> MSLPIRNSIKRYKEQLKKPLFKNEALYQLTKLYLSLENEINENELDECKDYFNQLKQSGVLKESQKELKEITIDFQTITKQYDLAEQSLQSAIKSYPDNLNFLLKNINLLSINKKYYEFFKSIKDSKIKYQRDLKYLNFIIKQIDNVAIKAIKESVEEIQANTMLLNDSMSYLNLITLKTEILDYIIRATIHNNLVSSNSSGSIDDIDDIGDYYGNNNFNQKLTRQLKEFKKQVKKIRELVSLYKEPITLSPSLEEFNERYFFYKGILIDYEYSNISNITTSISNIKNRQNPPFKSYLKSLQKDITKSSSSNMLEPIVKLSSEVSRQLFYSINRIIGDGNEIDLKLNFYASLNNNINMNLNIGDSGMYKYLDYLVSKFNSVSSPNDTDQLDTLFIESIEKNDFQYLLNNPLEFQRFISFSLWHINKTSSYTTLICWLDKIFNKFINRINFELQQLSSKSSSSTTTTTTSSSSHITLLHIIVYCINLIFETDYQQDYQQQQKQQQQQQQQQSYQLSSLEVYLDSTLNVPFLRNSLPWKIWNSMIYYSNLKPSSKINSTEIFSITTLSELLNGILKNGDHLHPLTCYKIAKDLPMITQHYQNEVDLSQTDIDISKIQATYYLITLRHITYLNQQRQQQQQDNNNNNDINNNNNNNNQIIQDKNFLKNIENTCNHCLSDLYKDKQNLKGALQYLLKVDTPIAYVETIYLCRDIIYNNKSNPAYTRPVIQSLITLMNQVWNKCQDFNANDLDYYQVDHDEYLNDIDASLEIITKLKDQYNFYDVPSTPSSSSLYTTPTKPTTVVPFSSIYGNNYNNNNNNNNNSLISSTPQRGRLSLPSTSTPLKVSMLSNSPNKSNNNNNNNNKQIQQSQQNKSDLPKFNVVEEEEEEEEVDINSFKDVFLQRRKERAELLKTLSNKRKALVCPQEFNKPLRSLDYVPPEGTVITKPTVVPTTTTSPIQTNSAFFGTTTPNSLLVNPVVPLPTTSTSPPSLFGVTTTTTTTSPTSLFGKTNTSPSSIFGTTPTSTSTSTAPLFGTSAPTSSLFGTTASSTPSTTATPATPFSTTATSTPSTTTTPATPFSTTATTTPNIFGSTLTTGLFGTKTPTSVSLPQSISTPTLADKTIKTEESTTSVSPPPPPPLPTKSNTPTKPATITPTTSNATSSSSSMSSIFANASVNASSMFGNTSSSSSIFGTPSSQTFGSISSPTSNLGSLFGGTKDFKPVETTTITTATSPPSISENKSTTTSDTNKPVETTTTTTATSPPSISENKPITTSDTNKPVETTTSNTLFGATTTTTGLFGLTKTSNTATGISLFGNSSSILNSSLLSKKDGSSDEDSDEDSDEQDSEEDSEEEKGKTTKSNSSLQRKKNEVSHKKDSKNRLQTLKDKISKKNNNNNTQKDIIKPQQQKQQTSQSSKNLSDDDQDEEYESQEEDENQDDDQANEEYDEDDYEEEDEDYEEDEEDEDEEEEEEEDYKEDPNKPKPTFLFGTSSTTSNPAQTTTPTTSTPTPSSSIFGQPPTSSSVFGSKPTVFGSASSNSSSVFGQTTTKPSTGSSVFGQNSSSVFGQTTTPSSGTGVFGQNSSSVFGQTSTGTGVFGQNSSSIFGQSNGVMGSTSTPSSTSIFGVKKSDELTKKTEESVKKTEESASSTTPSKLIWKCLCCENENSEKEKSCSVCMVPVPKNVKFESPASESNTKPSLIAPTAFGSNVTQTSTPLGKLIWKCLCCETENLEKETSCSVCMVPLPKNVKFESPASESNNKPSSLFAPTAFGGNAPPTTSTAVESSKLFGGGGITFNAPNIFGNNSNPSNLFGSGNNNSSSLFGGNSTTNPPPLFGNKSDVKTEESEKKAEASTPSPSTTSGKLIWKCLCCETENSEKEKSCSVCMVPVPKNVKFESPASESNTKSSLFAPTAFGGNAPPTTSTAVESSRLFGGGGGNGITFNAPNIFGNNNNPSNLFGNGNNNSSSLFGGNSTTNPPPLFGNKSDVKIQESEKKAEESEKKANESTPSPSTSTPSGKLIWKCLCCETENSEKEKSCSVCMVPVPKNVKFESPASESNTKSSLFAPTAFGGNAPPTSTAVDSSKLFGGGGGGSNTITFNAPNIFGNNNNNTSNLFGSGNSTSTPLFGTKPTETKAEVKAESKTESNVEETAPSSTSTPSGKLIWKCLCCETENSEKEKSCSVCMV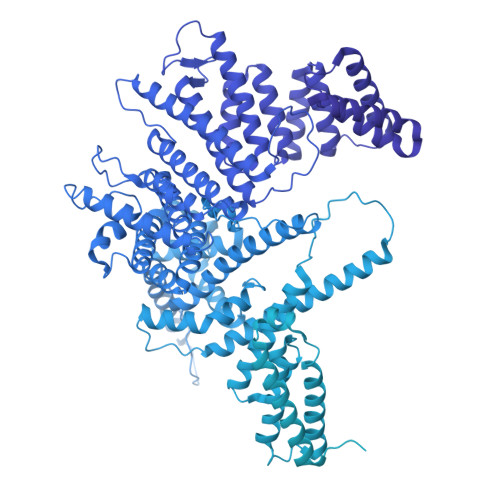PLPKNVKFESPASESNTKPSSLFAPTAFGGNAPPTSTAVESSKLFGGGGGNTFNAPNLFGNNNTSNLFGSGNSTSTPLFGTKQTEIKTEVKAESKIESKVEETAPSSTSTPSGKLIWKCLCCETENSEKEKSCSVCMVPLPKNVKFESPASESNTKPSSIFAPTAFGGNAPPTTSTAVDSSKLFGGGGSNTITFNAPTLFGNNNNSNPSNLFGSGNNNSSSLFGGNSTTIQPSQSLFGTKSTETKSDDPMSLKEMSNTIQDNDDQNSDSESHEELESGSEEEEEQQQQPKVTLLSSSFTPPSFAPPSFAPSSFAPSSFAPPSFAPPSFAPSSFAPSSFAPPSFAPPKPENTSTPTSSIFGSFSSQPSGGGISAFGPVSSNSSSPFGSGFGSASIPSFGQSQVNPLTINPTSTSPTAVFGGSTTSQFSSSSPAPIFGSTATIKTFGDLSKPSLSNNENKDQTSSSPSKPSPSPSNPTFESINKEKESVEDKNQEKDELKDEKDELKDENEKKDENEKKEETVESDKEKEKEETLEETKQSIESDKKEEKKEEKLEEIVQSDKEKEKEETLEETKQSIESDKKEDEKEEKLEEIVESDKEKEKEETLEETKQSIESDKKEDEKEEKLEEIVQSDKEKEKEETLEEIKQSIESESDKKEDEMEKVFSRIEETIKPNFFSTKEDEEEKGDELKDEKDENENEIESDNEKEKEETLEETKQSIESDKKEDEKEETLEEIVQSDKEKEKEETLEETKQPIETDKKEDEKENETEPEKHIDNEKKDENEKKNEDEKKEEETVESDQEKEKEETKQSIESESDKKEDEMEKEFSRIEETIKPNFFSTNKDEKDQETKEDNGNSDNNIDQETKENEKASKEIQDEEEEKEKEQEEPNLSLLSMDPVRCMSLSGLPIFDQTVKVEEEIEYEKDDGDDDDDDETIEKDSSSTTTSTTTTSTTTASTLTPQKPLFAPSSFAPPSFSLPTPTIQASSIFGSFSSQPSGGGISAFGPVSSNSSSSPFGSAFGSSFGSTTIPSFGQSQVNPLTINPTSTSPTPVFGGSTTSQFSSSSPAPIFGSTATIKTFGDLSKSSSSNNENKDQPSSSPSPSKPTSESTTKEEKVDIVEDKTDKIEENKEDSEDEKVITEDTNNQSEIKVEENKEENKEENKEENKEENKEEEKEEEKRIKQQQQSIESESDKRENEMEDKFSKIEELVKPDFIPCKVEEKLSEEQTKENIDNNDDNNTTSSIVVQENTTETISENDNDQSIQLDSNKQEIKKSIESESDKKEEVMEKNFTEIENLVKPNLMNSTQEEQQNQENKVEKEEENVNKTEEKEEDENLEKQNQTIEKENEEISELKDIQENNENNEESSTSSDGEESKSIKDVDTSYDDVD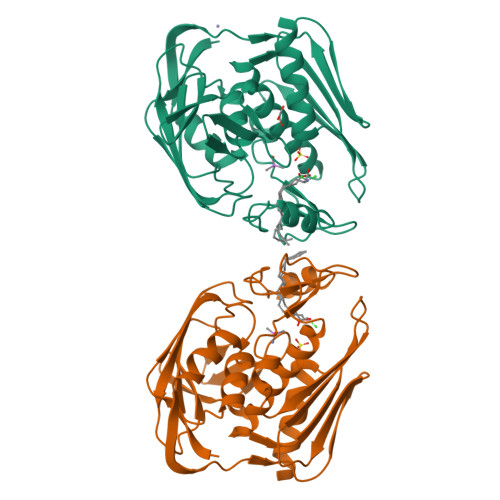>[2x]GLEKTVKEKLSFEGVGIHTGEYSKLIIHPEKEGTGIRFFKNGVYIPARHEFVVHTNHSTDLGFKGQRIKTVEHILSVLHLLEITNVTIEVIGNEIPILDGSGWEFYEAIRKNILNQNREIDYFVVEEPIIVEDEGRLIKAEPSDTLEVTYEGEFKNFLGRQKFTFVEGNEEEIVLARTFAFDWEIEHIKKVGLGKGGSLKNTLVLGKDKVYNPEGLRYENEPVRHKVFDLIGDLYLLGSPVKGKFYSFRGGHSLNVKLVKELAKKQKLTR> SNAFEEVRDFFYDRNNYIHDLDMAAERMFTESGMRTGGLDIQLAELMRDRFGISVVIDDNLPDTAKRRYHPDTKVLRVAHWLMPGQRAFQIATQLALVGQSDLISSIVATDDQLSTEARGVARIGLANYFAGAFLLPYREFHRAAEQLRYDIDLLGRRFGVGFETVCHRLSTLQRPRQRGIPFIFVRTDKAGNISKRQSATAFHFSRVGGSCPLWVVHDAFAQPERIVRQVAQMPDGRSYFWVAKTTAADGLGYLGPHKNFAVGLGCDLAHAHKLVYSTGVVLDDPSTE

Upregulation of the methylcitrate cycle (MCC) is required to assimilate and detoxify propionyl-CoA, a cholesterol degradation product. The transcription of key genes prpC and prpD in MCC is activated by MtPrpR, a member of a family of prokaryotic transcription factors whose structures and modes of action have not been clearly defined. We show that MtPrpR has a novel overall structure and directly binds to CoA or short-chain acyl-CoA derivatives to form a homotetramer that covers the binding cavity and locks CoA tightly inside the protein. The regulation of this process involves a [4Fe4S] cluster located close to the CoA-binding cavity on a neighboring chain.

We then truncated a large portion of the C-terminal region (residues 441–486) containing the 447C-X2-C-X4-C455 iron-sulfur cluster-binding motif. In addition, residues 81–154, which were not visible in the MtPrpR81–486 structure due to flexibility, were also removed from the expression construct. The resultant prpR155–440 expression construct produced soluble protein with no color and the protein was a monomer in solution as shown by SEC. The crystal structure of MtPrpR155–440 showed that the protein retained the DIII-GAF core structure of MtPrpR81–486 and, as expected, had no bound [4Fe4S] cluster. However, CoA was also absent in the structure, even though 1 mM CoA was incubated with the protein during crystallization. The iron-free structure revealed a dramatic conformational change of the protein. The loop between β7 and β8 of the GAF-like domain flipped back nearly 180 degrees to be oriented towards the CoA-binding cavity and blocked the cavity entrance. A hydrophobic fragment of the loop with the amino acid sequence of 402GLGYLGP408 inserted into the cavity, interacting with Phe240, Phe336, Phe412, Trp232, His319 and Val414, all within van der Waals distances to the loop. Gly404, Tyr405 and Leu406 at the tip of the loop occupy the space where the 3′-phosphoadenosine diphosphate moiety of CoA resided in the CoA-bound form of the protein. Taken together, the iron-sulfur cluster determines the ability of MtPrpR to bind CoA by regulating the conformation of this hydrophobic loop.>[3x]MGKKITILLGALLPFTSAVADEPALSPEAITSAQVFSTQSKETYTYVRCWYRTGNSHDESA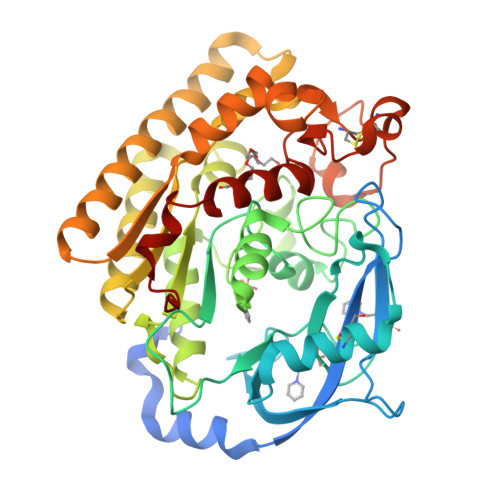TDWEWAENPDGSYFTIDGYWWSSVRLKNMFYTNTSQNVIKQRCEETLGVTHDAADITYFAADNRWSYNHTIWTNDPVMQADQINKIVAFGDSLSDTGNIFNAAQWRFPNPDTWFLGHFSNGFVWTEYIAQAKKLPLYNWAVGGAAGSNQYVALTGVKDQVLSYLTYAKMAKNYKPENTLFTLEFGLNDFMNYNREVVDVKTDFSTALIKLTDAGAKNIMLMTLPDATKAPQFKYSTQAEIEKVRAKIVEFNEFIKAQAAFYIIQGYNITLYDTHGLFEQLTQNPQQHGFVNASDACLNINRASSADYLYSHSLTNECATHSSDKYVFWNVTHPTTAVHKYIAEKMLAPGAGMQRFNFHHHHHH>MDPLTGLPNRRYFFELGNRYLDLAKREGKKVFVLFVDLAGFKAINDTYGHLSGDEVLKTVSKRILDRVARSDVVARYGGDEFTILLYDMKEEYLKSLLERILSTFREPVRV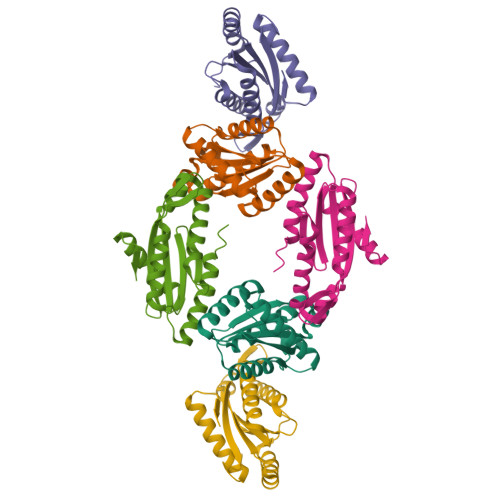ENKHLSVTPNIGVARFPEDGENLEELLKVADMRMYKAKEMKVPYFSLSLEHHHHHH[6x]>MKIIRIETSRIAVPLTKPFKTALRTVYTAESVIVRITYDSGAVGWGEAPPTLVITGDSMDSIESAIHHVLKPALLGKSLAGYEAILHDIQHLLTGNMSAKAAVEMALYDGWAQMCGLPLYQMLGGYRDTLETDYTVSVNSPEEMAADAENYLKQGFQTLKIKVGKDDIATDIARIQEIRKRVGSAVKLRLDANQGWRPKEAVTAIRKMEDAGLGIELVEQPVHKDDLAGLKKVTDATDTPIMADESVFTPRQAFEVLQTRSADLINIKLMKAGGISGAEKINAMAEACGVECMVGSMIETKLGI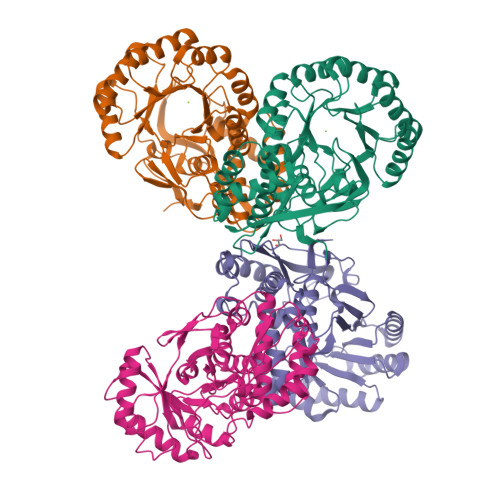TAAAHFAASKRNITRFDFDAPLMLKTDVFNGGITYSGSTISMPGKPGLGIIGAALLKGEKEQ[4x]>MNTFDKHDLSGFVGKHLVYTYDNGWEYEIYVKNENTLDYRIHSGLVGNRWVKDQQAYIVRVGESIYKISWTAPTGTDVSLIVNLGDSLFHGTIFFPRWVMNNPEKTVCFQNDHIPLMNSYRDAGPAY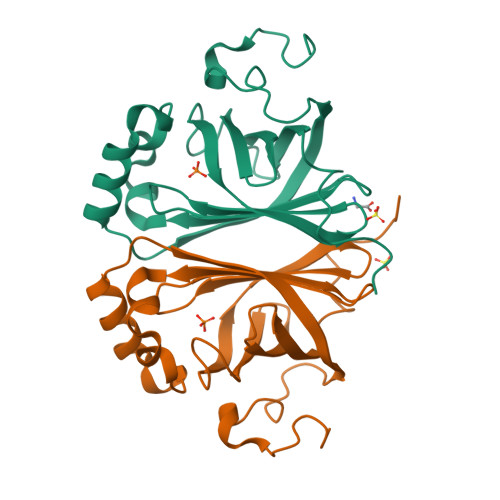PTEVIDEFATITFVRDCGANNESVIACAASELPKNFPDNLK[2x]> LECHNQQSSQPPTTKTCSPGETNCYKKVWRDHRGTIIERGCGCPTVKPGIKLNCCTT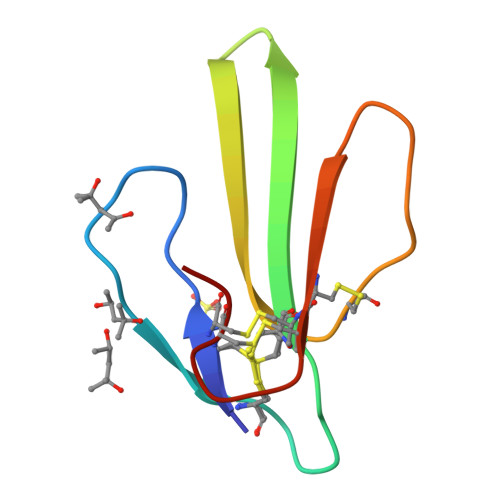DKCNN> IIANAVVAQDGTGDYQTLAEAVAAAPDKSKTRYVIYVKRGTYKENVEVASNKMNLMIVGDGMYATTITGSLNVVDGSTTFRSATLAAVGQGFILQDICIQNTAGPAKDQAVALRVGADMSVINRCRIDAYQDTLYAHSQRQFYRDSYVTGTVDFIFGNAAVVFQKCQLVARKPGKYQQNMVTAQGRTDPNQ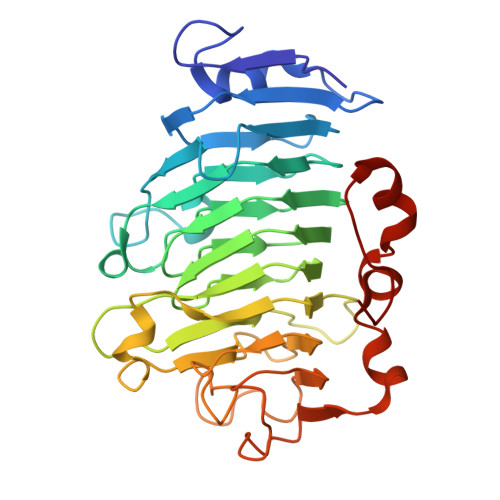ATGTSIQFCNIIASSDLEPVLKEFPTYLGRPWKEYSRTVVMESYLGGLINPAGWAEWDGDFALKTLYYGEFMNNGPGAGTSKRVKWPGYHVITDPAKAMPFTVAKLIQGGSWLRSTGVAYVDGLYD> QPIFLNVLEAIEPGVVCAGHDNNQPDSFAALHSSLNELGERQLVHVVKWAKALPGFRNLHVDDQMAVIQYSWMGLMVFAMGWRSFTNVNSRMLYFAPDLVFNEYRMHKS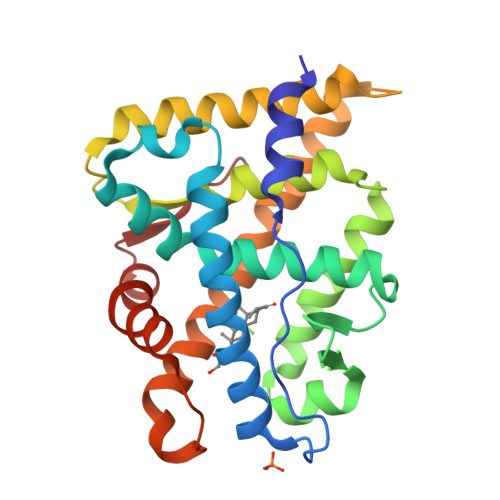RMYSQCVRMRHLSQEFGWLQITPQEFLCMKALLLFSIIPVDGLKNQKFFDELRMNYIKELDRIIACKRKNPTSCSRRFYQLTKLLDSVQPIARELHQFAFDLLIKSHMVSVDFPEMMAEIISVQVPKILSGKVKPIYFH Collagen-like peptides have been utilized as a molecular platform to investigate side chain interactions. The characteristic structure of a collagen-like peptide is a triple helix composed of three chains. Each chain adopts a well-extended PPII conformation with successive Gly-X-Y triplets. Chain trimerization is induced by inter-chain backbone hydrogen bonding between Gly and non-Gly residues.

In this study, in order to gain structural insights into an NH–π interaction between Gln and Phe and better understand its chemical properties, we solved a crystal structure of a collagen-like peptides (GPO)3GPQGFO(GPO)3, abbreviated as GPQGFO, and characterized the side chain interactions using several lines of evidence including circular dichroism, quantum chemical analysis, molecular dynamics simulation, and structural bioinformatics. The GPQGFO peptide crystallizes with the triple helical structure characteristic of collagen molecules with 1.385 Å resolution. Two axial pairs and one lateral were observed in the structure depending on the relative positions of the interacting amino acids. Two axial pairs were, respectively, composed of Gln in the leading and Phe in the middle chains of the triple helices, the other was between the middle and trailing chains. The conformations were located at the region with dNM ~3.3 Å, θ ~10° and ω ~150°, well within the empirical cutoffs for NH–π interactions (dNM < 4.3 Å, −25° < θ < 25°, and ω > 120°) extracted from the previous data-mining of protein structures. There was a third pair between Gln in the trailing and Phe in the leading chains. The side chains were pointed in opposite directions (dNM = 7.4 Å), which did not form any interactions. In the GPQGFO structure, Gln and Phe, with Cα atoms separated by 7.7 Å, made a strong NH–π interaction. The MD data suggested that the Q-F pairs in the crystal structure should be maintained in solution to stabilize the protein, consistent with the observations in the CD experiments. From thermal unfolding experiments, we have demonstrated that NH–π interactions allow the side chain of Gln to interact with the π-system of Phe in an axial geometry that is less influenced by the environment.

>[3x]XGPPGPPGPPGPQGFPGPPGPPGPPX>AFNDIKSKDATFASGTLDLSAKENSASVNLSNLKPGDKLTKDFQFENNGSLAIKEVLMALNYGDFKANGGSNTSPEDFLSQFEVTLLTVGKEGGNGYPKNIILDDANLKDLYLMSAKNDAAAAEKIKKQIDPKFLNASGKVNVATIDGKTAPEYDGVPKTPTDFDQVQMEIQFKDDKTKDEKGLMVQNKYQGNSIKLQFSFEATQWNGLTIKKDHTDKDGYVKENEK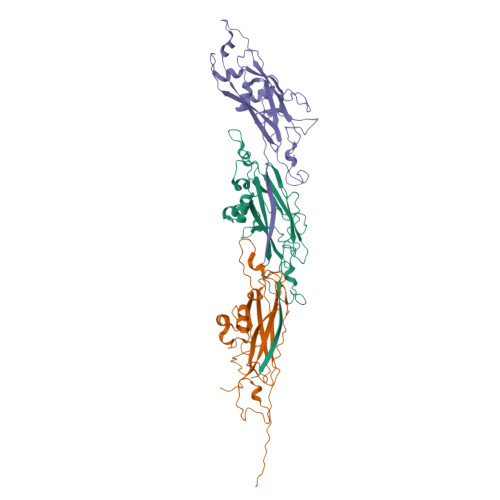AHSEDKN[3x]>GAMGASGKIKISTPYNLTKRMMMPMLNGFMSQYPEINIELTTESNADQLDPTEWDVIFRVGPQRDSSLIARKIGSVKDILVASPEYVNAHPMPTHAEDLHDHFLLKGHPLLKWTLINSKGETVVNVDRGRFQANALNVVRSASSEGLGITLMPDVMIKEYIADGSLVRILPDWSANPRDIYMLYNHKDHLPEKVRLFIDYVIAYNI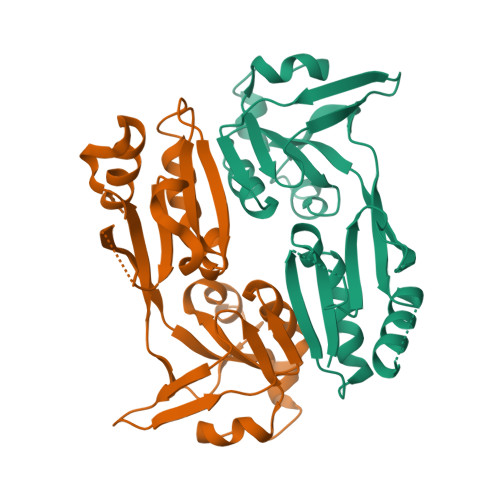H[6x]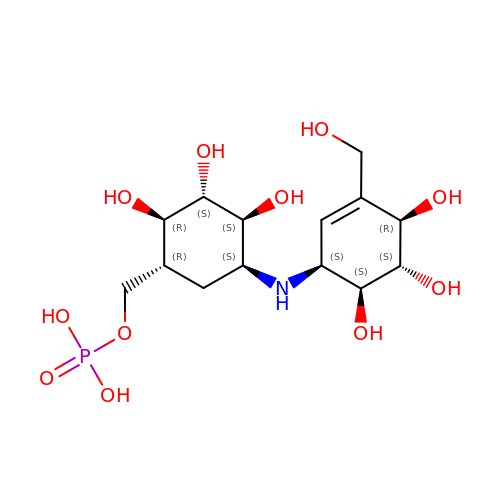[(1R,2R,3S,4S,5S)-2,3,4-TRIHYDROXY-5-{[(1S,4R,5S,6S)-4,5,6-TRIHYDROXY-3-(HYDROXYMETHYL)CYCLOHEX-2-EN-1-YL]AMINO}CYCLOHEXYL]METHYL DIHYDROGEN PHOSPHATE | C14 H26 N O11 P | ZKSTYMJGEHZSFH-MBABXGOBSA-N>SHMTPKELLEWQTNWKKIMKRDSRIYFD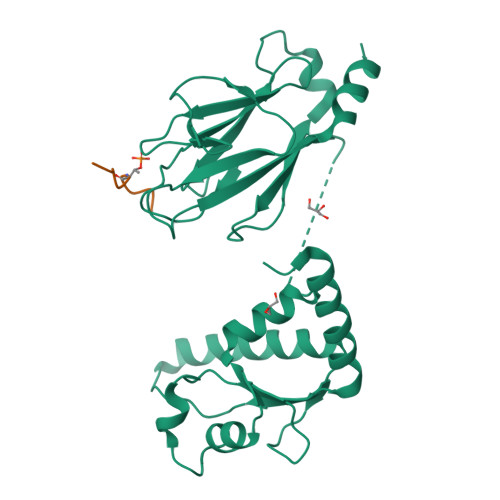ITDDVEMNTYNKSKMDKRRDLLKRGFLTLGAQITQFFDTTVTIVITRRSVENIYLLKDTDILSRAKKNYMKVWSYEKAARFLKNLDVDLDHVDGSKFSQEQIGENIVCRVICTTGQIPIRDLSADISQVLKEKRSIKKVWTFGRNPACDYHLGNISRLSNKHFQILLGEDGNLLLNDISTNGTWLNGQKVEKNSNQLLSQGDEITVGVGVESDILSLVIFINDKFKQCLEQNKVDR[2x];>[2x]DGESTDEDDVVS> DV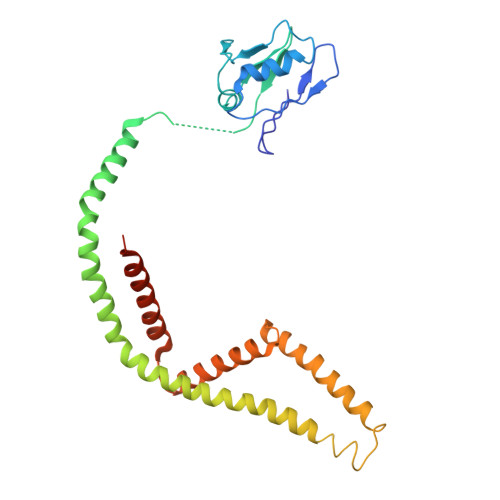TVVYQNGLPVISVRLPSRRERCQFTLKPISDSVGVFLRQLQEEDRGIDRVAIYSPDGVRVAASTGIDLLLLDDFKLVINDLTYHVRPPKRDLLSHENAATLNDVKTLVQQLYTTLCIEQHQLNKERELIERLEDLKEQLAPLEKVRIEISRKAEKRTTLVLWGGLAYMATQFGILARLTWWEYSWDIMEPVTYFITYGSAMAMYAYFVMTRQEYVYPEARDRQYLLFFHKGAKKSRFDLEKYNQLKDAIAQAEMDLKRLRDPLQVHLPLRQ>[2x]ARKREVRLMKNREAARECRRKKKEYVKCLENRVAVLENQNKTLIEELKALKDLYCHKSD;>MATSGANGP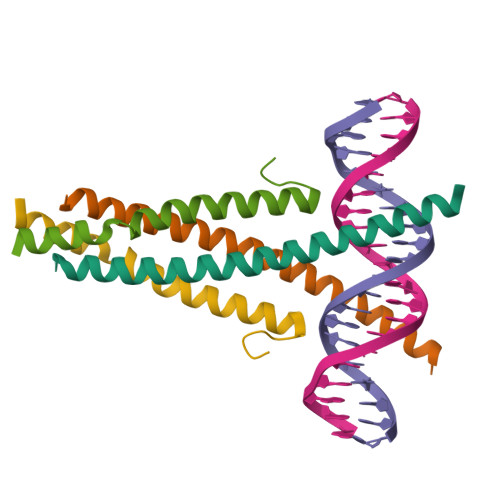GSATASASNPRKFSEKIALQKQRQAEETAAFEEVMMDIGSTRLQAQKLRLAYTRSSHYGGSLPNVNQIGCG[2x]> MGSDKIHHHHHHMSKLIVPQWPQPKGVAACSSTRIGGVSLPPYDSLNLGAHCGDNPDHVEENRKRLFAAGNLPSKPVWLEQVHGKDVLKLTGEPYASKRADASYSNTPGTVCAVMTADCLPVLFCNRAGTE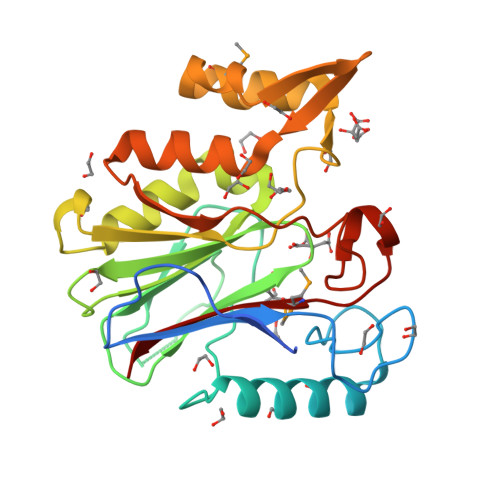VAAAHAGWRGLCAGVLEETVSCFADNPENILAWLGPAIGPRAFEVGGEVREAFMAVDAKASAAFIQHGDKYLADIYQLARQRLANVGVEQIFGGDRCTYTENETFFSYRRDKTTGRMASFIWLI>AMGSVTVHSSEP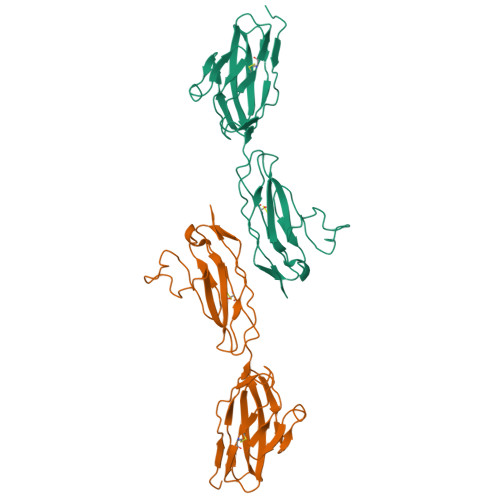EVRIPENNPVKLSCAYSGFSSPRVEWKFDQGDTTRLVCYNNKITASYEDRVTFLPTGITFKSVTREDTGTYTCMVSEEGGNSYGEVKVKLIVLVPPSKPTVNIPSSATIGNRAVLTCSEQDGSPPSEYTWFKDGIVMPTNPKSTRAFSNSSYVLNPTTGELVFDPLSASDTGEYSCEARNGYGTPMTSNAVRMEAVE[2x]> GPMQNEYIDAKKHGIDLSRERAPNFVDHPG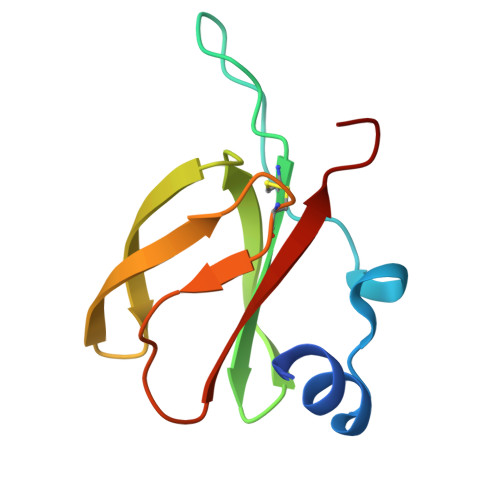IPPSDCFWFLYKNYVRQNAGVCQSDWSFDMKIGQYWVTIHTDEGCRLSGIIPAGWLILGMKRPGF> MANRSHHNAGHRAMNALRKSGQKHSSESQLGSSEIGTTRHVYDVCDCLDTLAKLPDDSVQLIICDPPYNIMLADWDDHMDYIGWAKRWLAEAERVLSPTGSIAIFGGLQYQGEAGSGDLISIISHMRQNSKMLLANLIIWNYPNGMSAQRFFANRHEEIAWFAKTKKYFFDLDAVREPYDEETKAAYMKDKRLNPESVEKGRNPTNVWRMSRLNGNSLERVGHPTQKPAAVIERLVRALS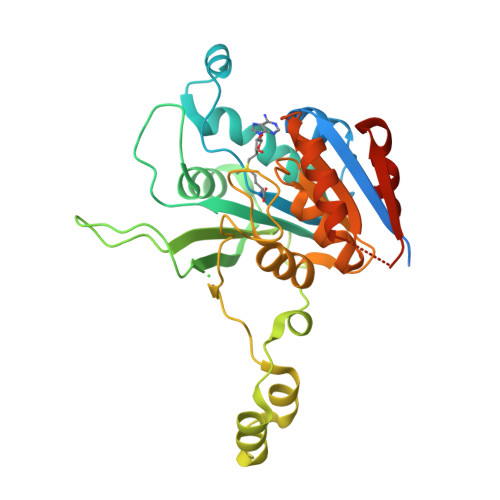HPGSTVLDFFAGSGVTARVAIQEGRNSICTDAAPVFKEYYQKQLTFLQDDGLIDKARSYEIVEGAANFGAALQRGDVAS>[2x]MQKSDEVTEKFKRYCNQLEKYGQTENVHSPVMAMLRRKGRKQLIEIMKRDGDCTSSINKLWIVGYYHPFQFFIRDKEKNMAIAVLLTMFCGELQEMLSLPDDKYPALWNMYIGDFHRYMPDEEIQKCLAVGYYSR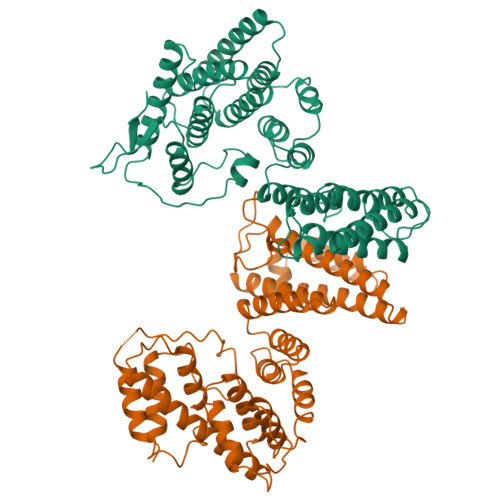AIDLDPNQGRAFHVLAGLRADLNVAQKLRLMILGQLADAPYKKGTELLEYLKFPQKESTDKLMVDFVIWALNEKSKRMDYQMTGIKIVNEFKAEIEQKLEFDWSLIMSTCRLASKLAMKKFGFQQFYNCFDTISTLYITIYSRTISSKCLLAEAISWISDSAEILGHLDEQKNEPHFQKLSVFAKTKWNELNDLVMNHINSVFTSMSLTINPSISMTSFLLNGPISEPNVEFLSQLINYLVSVEFPPMEIIHDREESGPLLRRINQSEQKRLDIQIKTQNDEVNR;>[2x]MSDEWEQLTVELRKIPRGTEAAPQYLRHLMKMFVADFETAVSKRFDVKFWNKLKSMMDEITKAMENDRLVNHNVQNLAIGFLTDLSLLVHYHYEIPNYGNDISKQLTWTPDVFLNRKPIKSKKNSRVFMAYVLLRMGDLMRYKENYPKAQEYYEQSCRINPADGAVWNQLGLISSLGAKNLESVYFHTRALHATMEFPTASGGLTNIFKNFANRDISRPMPIKDLYLSCLGRIHFLLEIEDSSVHLQKIGEEAATSKEMIVPLMSVYKHLEDGTELEQRAVEYVKTIWCTAYRSLLKTLDDYKEESKKLADVPHLLHILALLLCAPKLLRGIEDQTEDEVTSICEWLLCANCDEKIKDSDAFGYFHCLQRIQYPLTRTQLAQKLVEIEDEDESKD> MANKPTQPLFPLGLETSESSNIKGFNNSGTIEHSPGAVMTFPEDTEVTGLPSSVRYNPDSDEFEGYYENGGWLSLGGGGIRWETLPHAPSSNLLEGRGYLINNTTGTSTVVLPSPTRIGDSVTICDAYGKFATYPLTVSPSGNNLYGSTEDMAITTDNVSATFTWSGPEQGWVITSGVGLGQGRVYSREIFTQILASETSAVTLNTPPT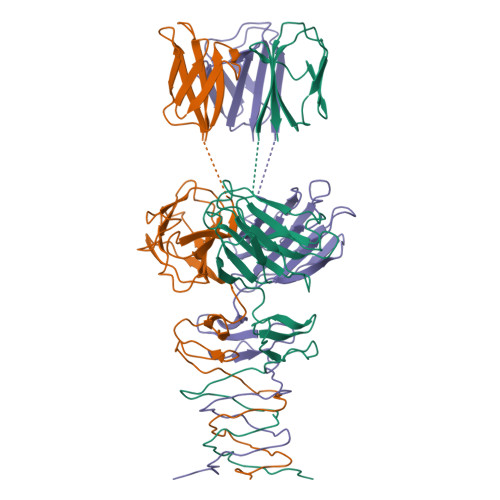IVDVYADGKRLAESKYSLDGNVITFSPSLPASTELQVIEYT1-O-{6-chloro-5-[4-(1-hydroxycyclobutyl)phenyl]-1H-indole-3-carbonyl}-beta-D-glucopyranuronic acid | C25 H24 Cl N O9 | 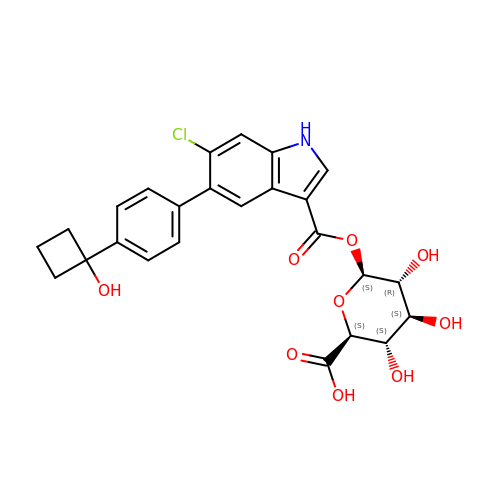LTLTUJCGZGVBTO-DCIKREJASA-N> SNAMTFNQEQDYWAGYKANERALIIQTWSGFGRYAPDHLYPPHILPLDTDNETLGTTVLQALANSRTFVYDSPEDQDFFDTEKIRQRYE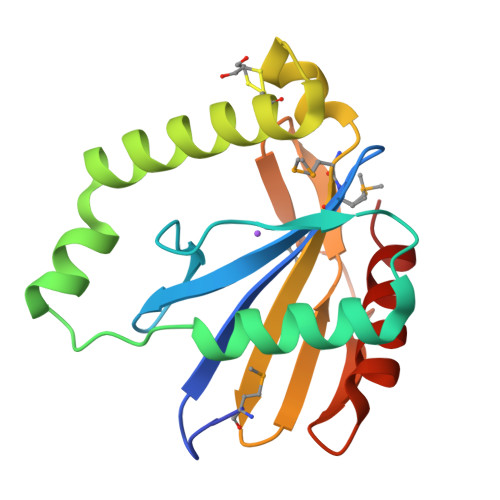DWVAKLCGNLGYKTRRALFKNMMSVDIWLHNGCLKISPSRHVKLEAWDAIDADDVILSLDNSPEEIGAGLKLALSRCR4-methyl-6-[2-(5-{4-[(methylamino)methyl]phenyl}pyridin-3-yl)ethyl]pyridin-2-amine 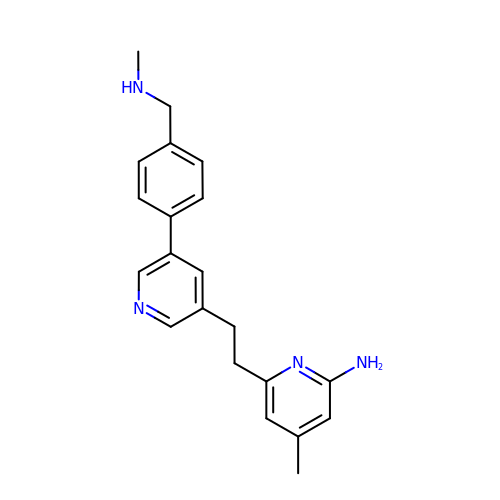| C21 H24 N4 | DWEUCJPXVJGNQN-UHFFFAOYSA-N>[3x]MGSSHHHHHHSQDPVSGTPDDGDIGLIIAVKRLAAAKTRLAPVFSAQTRENVVLAMLVDTLTAAAGVG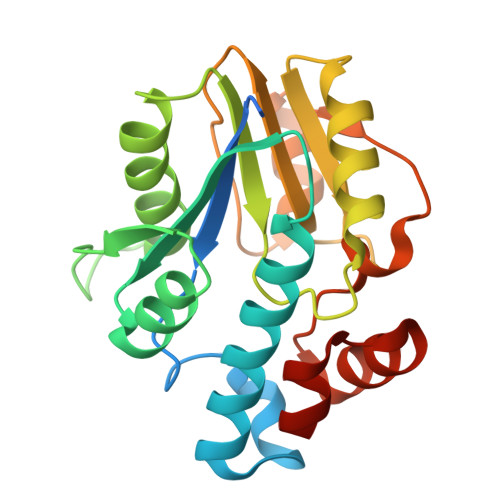SLRSITVITPDEAAAAAAAGLGADVLADPTPEDDPDPLNTAITAAERVVAEGASNIVVLQGDLPALQTQELAEAISAARHHRRSFVADRLGTGTAVLCAFGTALHPRFGPDSSARHRRSGAVELTGAWPGLRCDVDTPADLTAARQLGVGPATARAVAHR> VVGGTDADEGEWPWQVSLHALGQGHICGASLISPNWLVSAAHCYIDDRGFRYSDPTQWTAFLGLHDQSQRSAPGVQERRLKRIISHPFFNDFTFDYDIALLELEK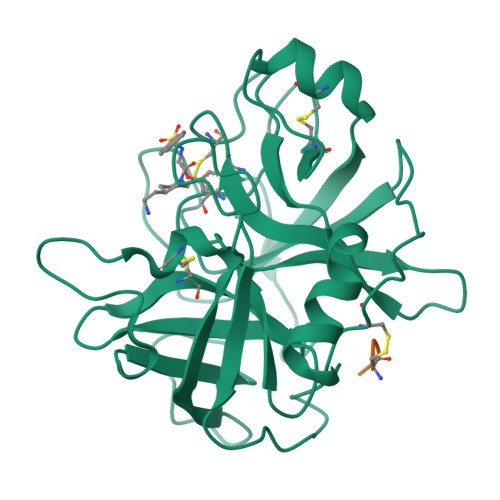PAEYSSMVRPICLPDASHVFPAGKAIWVTGWGHTQYGGTGALILQKGEIRVINQTTCENLLPQQITPRMMCVGFLSGGVDSCQGDSGGPLSSVEADGRIFQAGVVSWGDGCAQRNKPGVYTRLPLFRDWIKENTGV;> CGLR>[2x]SMSNNTVSTKPALHFLDINATEVKKYPTAIQDIIINRSFDGMIIRGVFPRDTMEQVARCLEEGNDGGMKSILNKNEEFGTKVAQIYGHAIVGQSPDLKDYFASSAIFRQACRTMFQGSPDFEEQVESIFHSLSGLPVEIPTGPEGQTYTPATIRLLLEGREIAVHVGNDFLLMPAANHLKTLLDLSDQLSYFIPLTVPEAGGELVVYSLEWNPQEASKYA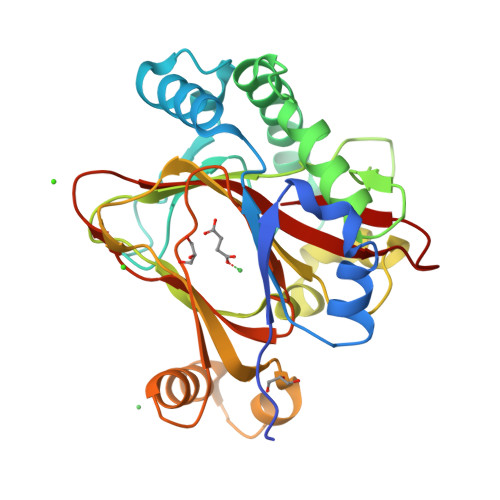QMQEYMDDVEFKIKSNQSQSVAYAPGPGDMLLFNGGRYYHRVSEVIGNSPRRTIGGFLAFSKQRDKIYYWS> S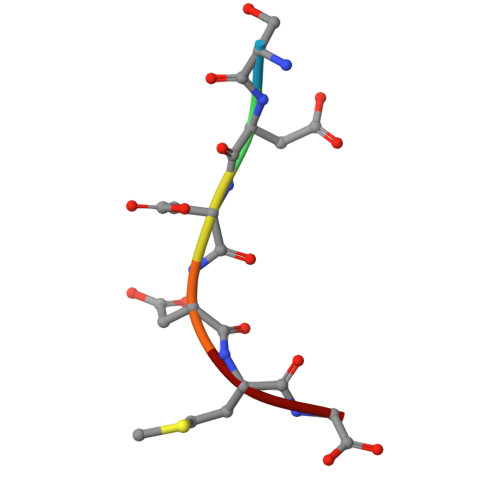DDDMG> CATCTAGCTCGTGGACTGAT;> TCATCAGTGGCAGT;> GAACTGCCTGAATTAC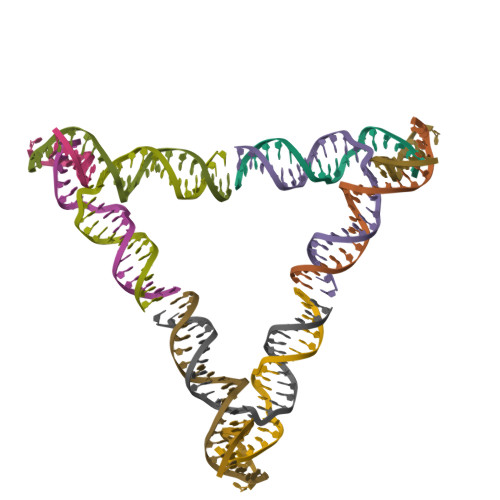TGACCG;> CGGTCAGTAATTCACCACGAGCTAGATG>[2x]MHHHHHHENLYFQGMPNVRNPFDLLLLPTWIVPVEPAGVVLRDHALGIRDGQIALVAPREQAMRHGATEIRELPGMLLAPGLVNAHGHSAMSLFRGLADDLPLMTWLQDHIWPAEGQWVSEDFIRDGTELAIAEQVKGGITCFSDMYFYPQAICGVVHDSGVRAQVAIPVLDFPIPGARDSAEAIRQGMALFDDLKHHPRIRIAFGPHAPYTVSDDKLEQI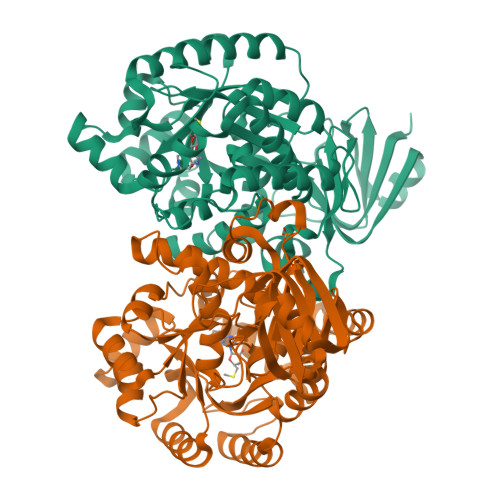LVLTEELDASIQMHVHETAFEVEQAMERNGERPLARLHRLGLLGPRFQAVHMTQVDNDDLAMLVETNSSVIHCPESNLKLASGFCPVEKLWQAGVNVAIGTDGAASNNDLDLLGETRTAALLAKAVYGQATALDAHRALRMATLNGARALGLERLIGSLEAGKAADLVAFDLSGLAQQPVYDPVSQLIYASGRDCVRHVWVGGRQLLDDGRLLRHDEQRLIARAREWGAKIAASDRS>MDYKDDDDKGDYKDDDDKIDYKDDDDKGSMADADGGSNLAVLDALDSARTQMYHMKAIVIAGMGFFTDAYDLFCISTVSKLLGRLYYQPDGSTDSKPGALSKTANNMVIGVALVGTLMGQLVFGYFGDKLGRKRVYGVTLILMAACAIGSGLSFGSSRKAVIGTLCFFRFWLGFGIGGDYPLSATIMSEYSNKKTRGAFIAAVFAMQGVGIIFAGLVSMIVSSIFLTYNKAPSYKGNHDLSRQMPAADYVWRIVLMIGAFPALATFYWRMKMPETARYTAIIDGNAKQAANDMQKVLSIEIEAEQEKLAKFNAANNYPLLSMEFARRHGLHLIGTTTTWFLLDIAFYSQNLTQKDIFPAMGLISGAAEVNALTEMFQISKASFLVALLGTFPGYWVTVALIDKMGRYMIQLIGFFMMSMFMLAMGILYDYLKTHHFLFGLLYALTFFFANFGPNST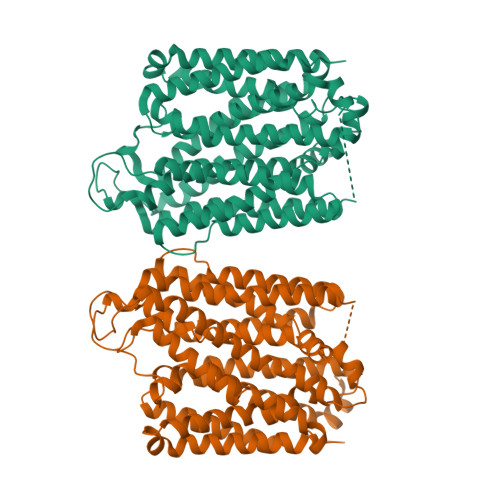TFVLPAELFPTRVRSTCHAISAAAGKAGAIVAAFGIQKLTYNSQVKSIKKALIILSITNMLGFFFTFLVPETMGRSLEEISGEDGNTGAGGGGAPAAANAGVGVSASDVSRDEKFPASSTEWQTSMHA[2x]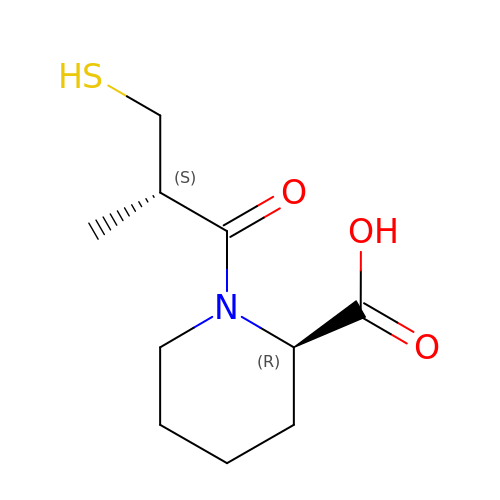(2R)-1-[(2S)-2-methyl-3-sulfanyl-propanoyl]piperidine-2-carboxylic acid | C10 H17 N O3 S | FFNRAOIWXHDKFF-HTQZYQBOSA-N2-acetamido-2-deoxy-alpha-D-mannopyranose 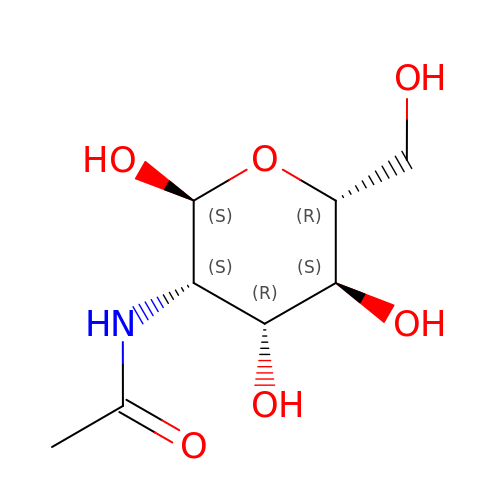| C8 H15 N O6 | OVRNDRQMDRJTHS-UOLFYFMNSA-N>EDADKLPHTKVTLVAPPQVHPHEQATKSGPKVVEFTMTIEEKKMVIDDKGTTLQAMT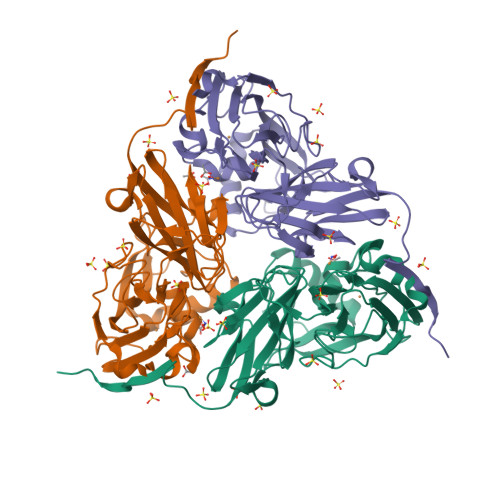FNGSMPGPTLVVHEGDYVQLTLVNPATNAMPHNVDFHGATGALGGAKLTNVNPGEQATLRFKADRSGTFVYHCAPEGMVPWHVVSGMSGTLMVLPRDGLKDPQGKPLHYDRAYTIGEFDLYIPKGPDGKYKDYATLAESYGDTVQVMRTLTPSHIVFNGKVGALTGANALTAKVGETVLLIHSQANRDTRPHLIGGHGDWVWETGKFANPPQRDLETWFIRGGSAGAALYTFKQPGVYAYLNHNLIEAFELGAAGHIKVEGKWNDDLMKQIKAPAPIPR[6x]>[4x]SALKEIQEAYILSGARTPTAKFNGSF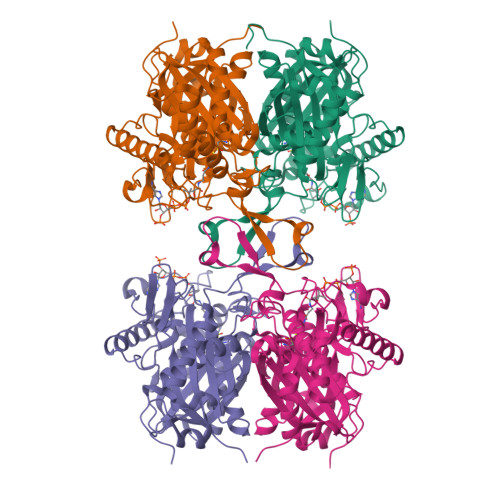VSVSAPELGAVAIKSAVSKSGVPVEKITDVYMGNVLQGAVGQAPARQASMFAGLSPTVESMTVNKVCASGLKAVALAAQNIQLGLAEAQVAGGMENMSRVPYYLPRSTQLPPFGEIKLQDGLIQDGLWDVYNQFHMGICAEKTAKKYEISREEQDQYAIQSYQRAQAAWKENKFAEEIAPVTVKGKKGETVVERDEGYENLRIDKMATLKPAFLRDGTGTVTAGNASTMNDGASALVLGSKAIAREFAQGNRALARIVSTADAAIDPVDFPVAPAKAVPIALERAGITKDQVAVWEFNEAFAAVIKANEKILGLQNARVNPLGGAISLGHALGSSGSRILVTLLHQLQPGEYGVAAICNGGGAATAMVVQKLDRVD>[2x]MASQSSVAVISSAAARGESFPDSKKPIGSVRFQQPLRLSFSYCKSGNMSSRICAMAKPNDAETLSSSVDMSLSPRVQSLKPSKTMVITDLA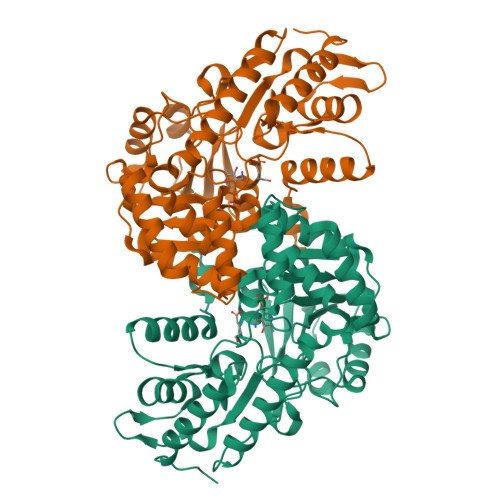ATLVQSGVPVIRLAAGEPDFDTPKVVAEAGINAIREGFTRYTLNAGITELREAICRKLKEENGLSYAPDQILVSNGAKQSLLQAVLAVCSPGDEVIIPAPYWVSYTEQARLADATPVVIPTKISNNFLLDPKDLESKLTEKSRLLILCSPSNPTGSVYPKSLLEEIARIIAKHPRLLVLSDEIYEHIIYAPATHTSFASLPDMYERTLTVNGFSAAFAMTGWRLGYLAGPKHIVAACSKLQGQVSSGASSIAQKAGVAALGLGKAGGETVAEMVKAYRERRDFLVKSLGDIKGVKISEPQGAFYLFIDFSAYYGSEAEGFGLINDSSSLALYFLDKFQVAMVPGDAFGDDSCIRISYATSLDVLQAAVEKIRKALEPLRATVSV> MQKLSRVVCNRLVRFHGTVAASAGGKRYDLFGYEVSVATGPFIEEIKKAQFYDDAGEVIVKMNLANTPPDLQTYNAVLERILNCKSKRSQPVKGENKFAAMMDILEEMDAR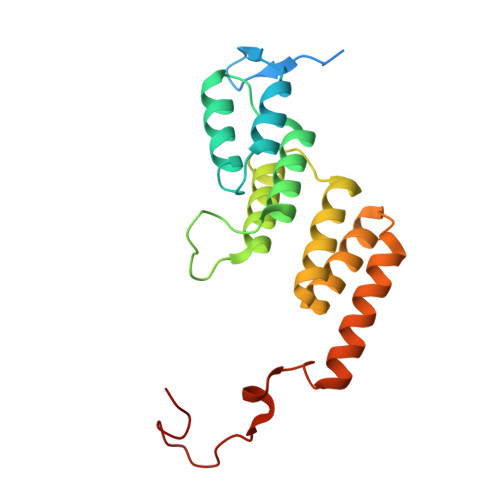SGIKPNAESWGYVLKELVQAGDFRLGWVCIAGMKSLGITPDQALVDANEANAAKAKAAGTDFPAYLKKAAPESFDTKAWGI> MRVVLIVDIVRQEEKLIAKALEENKVQYDIINVAQEPLPFNKALGRYDVAIIRPVSMYRALYSSAVLEA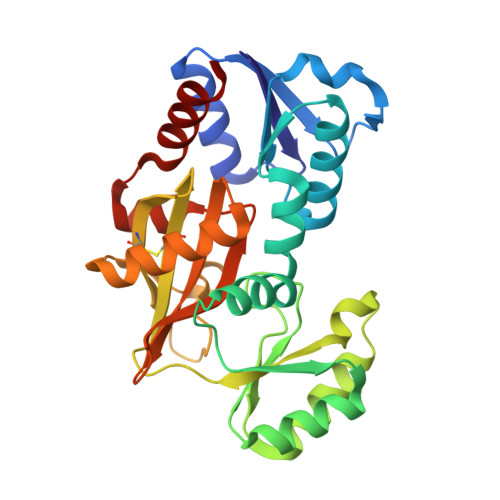AGVHTINSSDVINVCGDKILTYSKLYREGIPIPDSIIALSAEAALKAYEQRGFPLIDKPPIGSWGRLVSLIRDVFEGKTIIEHRELMGNSALKAHIVQEYIQYKGRDIRCIAIGEELLGCYARNIPPNEWRANVALGGTPSNIEVDEKLKETVVKAVSIVHGEFVSIDILEHPNKGYVVNELNDVPEFKGFMVATNINVAQKLVEYIKENYSK> MDRSGFGEISSPVIREAEVTRTARKQSAQKRVLLQASQDENFGNTTPRNQVIPRTPSSFRQPFTPTSRSLLRQPDISCILGTGGKSPRLTQSSGFFGNLSMVTNLDDSNWAAAFSSQRSGLFTNTEPHSITEDVTISAVMLREDDPGEAASMSMFSDFLQSFLKHSSSTVFDLVEEYENICGSQVNILSKIVSRATPGLQKFSKTASMLWLLQQEMVTWRLLASLYRDRIQSALEEESVFAVTAVNASEKTVVEALFQRDSLVRQSQLVVDWLESIAKDEIGEFSDNIEFYAKSVYWENTLHTLKQRQLTSYVGSVRPLVTELDPDAPIRQKMPLDDLDREDEVRLLKYLFTLIRAGMTEEAQRLCKRCGQAWRAATLEGWKLYHDPNVNGGTELEPVEGNPYRRIWKISCWRMAEDELFNRYERAIYAALSGNLKQLLPVCDTWEDTVWAYFRVMVDSLVEQEIQTSVATLDETEELPREYLGANWTLEKVFEELQATDKKRVLEENQEHYHIVQKFLILGDIDGLMDEFSKWLSKSRNNLPGHLLRFMT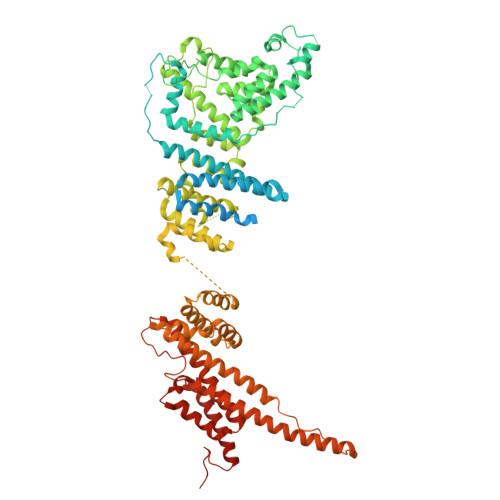HLILFFRTLGLQTKEEVSIEVLKTYIQLLIREKHTNLIAFYTCHLPQDLAVAQYALFLESVTEFEQRHHCLELAKEADLDVATITKTVVENIRKKDNGEFSHHDLAPALDTGTTEEDRLKIDVIDWLVFDPAQRAEALKQGNAIMRKFLASKKHEAAKEVFVKIPQDSIAEIYNQCEEQGMESPLPAEDDNAIREHLCIRAYLEAHETFNEWFKHMNSVPQKPALIPQPTFTEKVAHEHKEKKYEMDFGIWKGHLDALTADVKEKMYNVLLFVDGGWMVDVREDAKEDHERTHQMVLLRKLCLPMLCFLLHTILHSTGQYQECLQLADMVSSERHKLYLVFSKEELRKLLQKLRESSLMLLDQGLDPLGYEIQL> GSHMANKREPAPGWPIVSGEYVVGNPESCVGVVTLGSHGLEQACIDAGAAIAGPCHTENLGIEKVVANYISNPNIRFMILCGSEVQGHITGQCFKALWENGIGDDGGIIGAK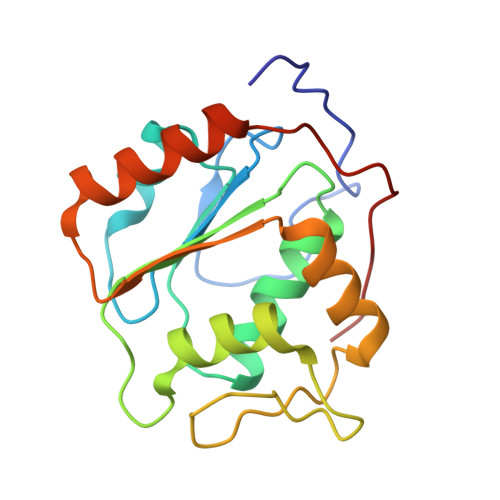GAIPFLENVNKEAVERFRRQIVEVVDLIDCEDIGKITQAIKECLSKDPGAIDEDPFIIELE> MALRNKAFHQLRQLFQQHTARWQHELPDLTKPQYAVMRAIADKPGIEQVALIEAAVSTKATLAEMLA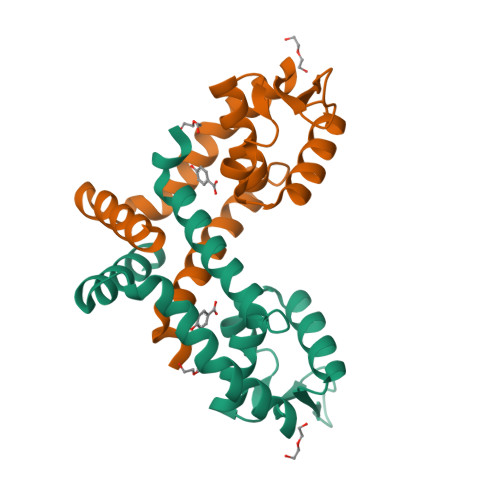RMENRGLVRREHDAADKRRRFVWLTAEGEKVLAAAIPIGDSVDEEFLGRLSAEEQELFMQLVRKMMNTLEHHHHHH> VIGVT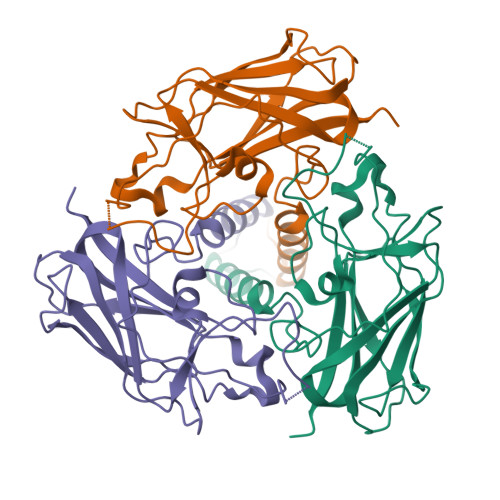EEQVHHIVKQALQRYSEDRIGLADYALESGGASVISTRCSETYETKTALLSLFGIPLWYHSQSPRVILQPDVHPGNCWAFQGPQGFAVVRLSARIRPTAVTLEHVPKALSPNSTISSAPKDFAIFGFDEDLQQEGTLLGKFTYDQDGEPIQTFHFQAPTMATYQVVELRILTNWGHPEYTCIYRFRVHGEPAHHHHHH>[2x]SGSMAAGERWWRFRVDYHAGPMDDLILDGVRPAFAAFAAQAPMAYFLRHWRRGPHLRIYVSTTREALEAVVRPAIEHVVGGYLRARPSPGMADPSAFLPLHERLAELEGEDGPLMPWSPDNTIHAEGERPEPLTVRDVLLADFYADTTPSVYHALERVRSGASLPTIAFD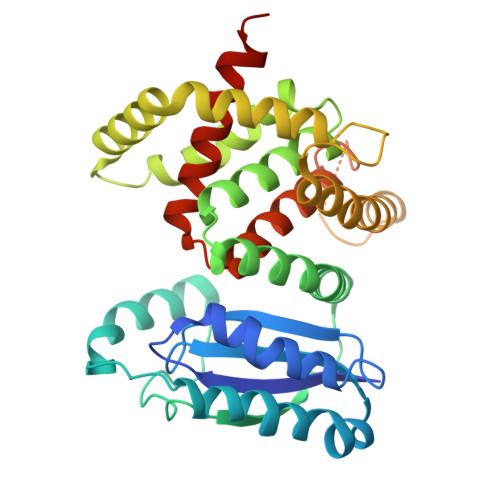LVVATAHALSTGGLPVARTSLRSHAEAYLARRSDGVRLRELWRDHYARNREAFTERLIAVASSAESAENGAHLPHVREWVRRLRPIRERARALLESGELTLEYASPAEGARDLPSLAEVSAFHRELESRPEWARLRDSPAFGAYRLVINCTYLHLTRLGLTPHQRFLVCHLAADAAADVYGIAAHEEVATR>PPGPPGPRGPPGPPGPPGGPGPPG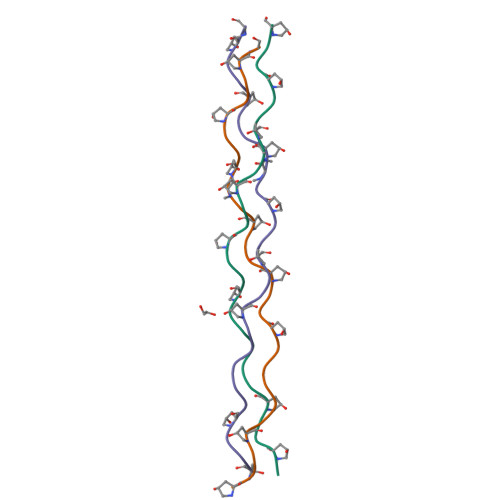PPGX[3x]> XGAQVSSQKVGAHENSNRAYGGSTINYTTINYYRDSASNAASKQDFSQDPSKFTEPI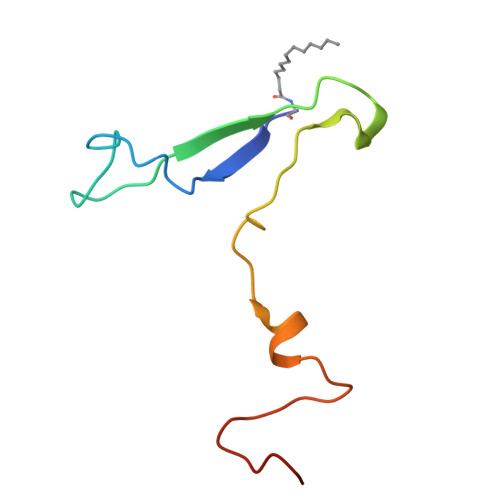KDVLIKTAPMLNS> MYEEFPDVITFQSYVEQSNGEGGKTYKWVDEFTAAAHVQPI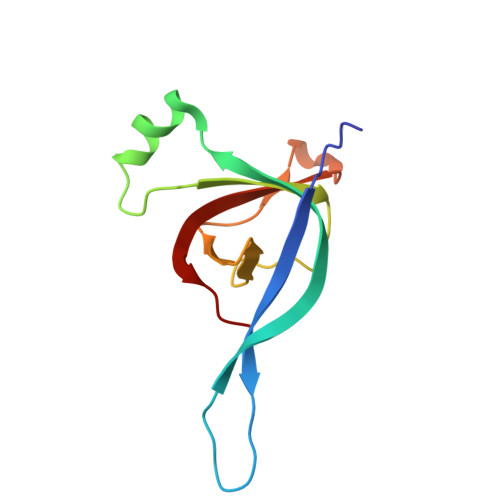SQEEYYKAQQLQTPIGYNIYTPYDDRIDKKMRVIYRGKIVTFIGDPVDLSGLQEITRIKGKEDGAYVG>GLIYGNYLHLEKVLNAQELQSETKGNKIHDEHLFIITHQAYELWFKQILWELDSVREIFQNGHVRDERNMLKVVSRMHRVSVILKLLVQQFSILETMTALDFNDFREYLSPASGFQSLQFRLLENKIGVLQNMRVPYNRRHYRDNFKGEENELLLKSEQEKTLLELVEAWLERTPGLEPHGFNFWGKLEKNITRGLEEEFIRIQAKEESEEKEEQVAEFQKQKEVLLSLFDEKRHEHLLSKGERRLSYRALQGALMIYFYREEPRFQVPFQLLTSLMDIDSLMTKWRYNHVCMVHRM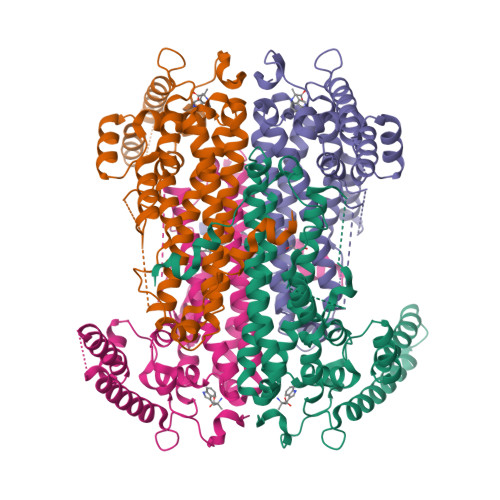LGSKAGTGGSSGYHYLRSTVSDRYKVFVDLFNLSTYLIPRHWIPKMNPTIHKFLEHHH[4x]> SGFRDRKVMEYENRIRAYSTPDKIFRYFATLKVISEPGEAEVFMTPEDFVRSITPNEKQPEHLGLDQYIIKRFDGKKISQEREKFADEGSIFYTLGECGLISFSDYIFLTTVLSTPQRNFEIAFKMFDLNGDGEVDMEEFEQVQSIIRSQTSMGMRHRDRPTTGNT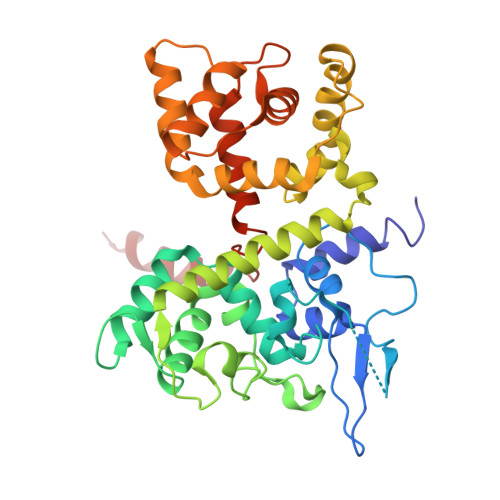LKSGLCSALTTYFFGADLKGKLTIKNFLEFQRKLQHDVLKLEFERHDPVDGRITERQFGGMLLAYSGVQSKKLTAMQRQLKKHFKEGKGLTFQEVENFFTFLKNINDVDTALSFYHMAGASLDKVTMQQVARTVAKVELSDHVCDVVFALFDCDGNGELSNKEFVSIMKQRLMRGLEKPKDMGFTRLMQAMWKCAQE> HSLFHX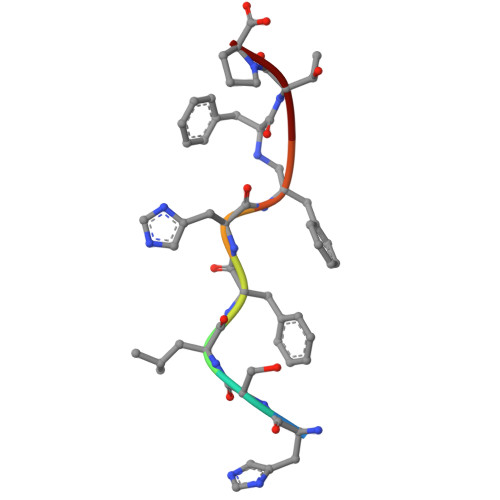TP>MDIKINDITLGNNSPFVLFGGINVLESLDSTLQTCAHYVEVTRKLGIPYIFKASFDKPRSSIHSYRGVGLEEGLKIFEKVKAEFGIPVITDVHEPHQCQPVAEVCDVIQLPAFLARQTDLVVAMA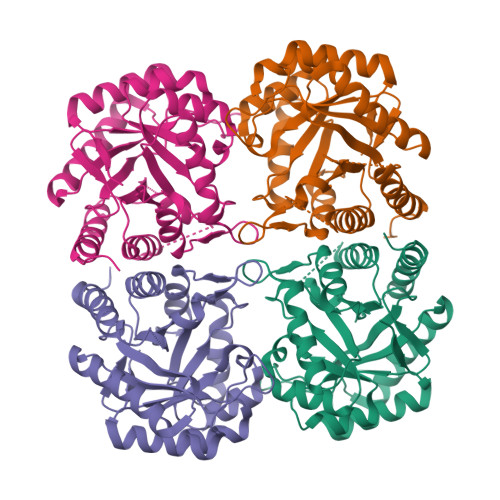KTGNVVNIKKPQFLSPSQMKNIVEKFHEAGNGKLILCERGSSFGYDNLVVDMLGFGVMKQTCGNLPVIFDVTHSLQTRDAGSAASGGRRAQALDLALAGMATRLAGLFLESHPDPKLAKCDGPSALPLHLLEDFLIRIKALDDLIKSQPILTIE[4x]> MGSSHHHHHHSSGENLYFQGHMIGSLGLVGSGEYLPALAEFEKSLIEDGIANGKKPIFLQIPTAAGRESENRIEFWKQLGRQQADRLGYESKFLPVLKREDADNPEFVELVKDAALIYFSGGDPHYLADTLINTPLWQGIYENWQ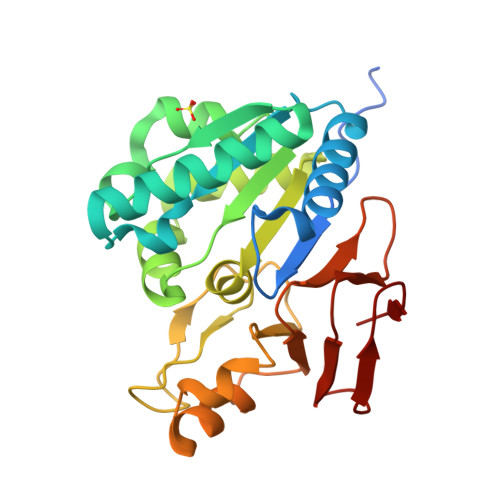SGGSLAGCSAGAMVLSTHVPNFRLSRHQSTEGFGIIENVRVIPHFNKFFKWIPDSAAKILLDLPTDSILIGIDEVTALVKRSGTDHWQVVGDAKVHILKGLPEQQLTAGESISF> GDITHMEKLGDICFSLRY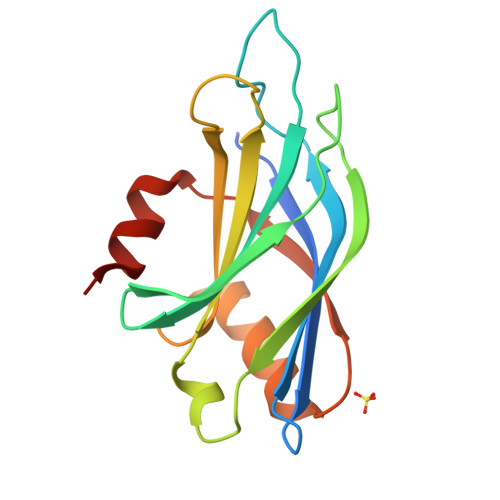VPTAGKLTVVILEAKNLKKMDVGGLSDPFVKIHLMQNGKRLKKKKTTIKKNTLNPYYNESFSFEVPFEQIQKVQVVVTVLDYDKIGKNDAIGKVFVGYNSTGAELRHWSDMLANPRRPIAQWHTLQVEEEVDAMLAVKK(2E,4E,6E)-3-methyl-6-(1,3,3-trimethyl-1,3-dihydro-2H-indol-2-ylidene)hexa-2,4-dienal 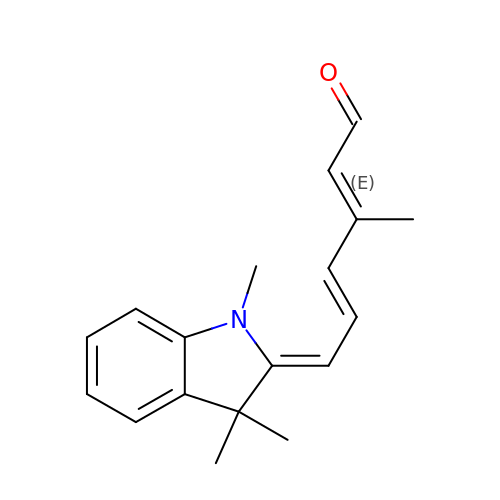| C18 H21 N O | UGINWNVBXWWHCS-RZZAMGAFSA-N>KAVIDIDAATKIMCSNAKAISLNEVEKNEIISKYREITAKKSERAELKEVEPIPLDWPSDLTLPPLPESTNDYVWAGKRKELDDYPRKQLIIDGLSIVIPTYNRAKILAITLACLCNQKTIYDYEVIVADDGSKENIEE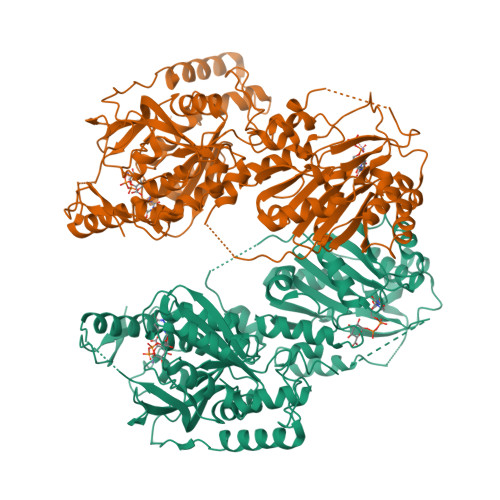IVREFESLLNIKYVRQKDYGYQLCAVRNLGLRAAKYNYVAILDCDMAPNPLWVQSYMELLAVDDNVALIGPRKYIDTSKHTYLDFLSQKSLINEIPEIITNNQVAGKVEQNKSVDWRIEHFKNTDNLRLCNTPFRFFSGGNVAFAKKWLFRAGWFDEEFTHWGGEDNEFGYRLYREGCYFRSVEGAMAYHQEPPGKENETDRAAGKNITVQLLQQKVPYFYRKKEKIESATLKRVPLVSIYIPAYNCSKYIVRCVESALNQTITDLEVCICDDGSTDDTLRILQEHYANHPRVRFISQKNKGIGSASNTAVRLCRGFYIGQLDSDDFLEPDAVELCLDEFRKDLSLACVYTTNRNIDREGNLISNGYNWPIYSREKLTSAMICHHFRMFTARAWNLTEGFNESISNAVDYDMYLKLSEVGPFKHINKICYNRVLHGENTSIKKLDIQKENHFKVVNESLSRLGIKKYKYSPLTNLNECRKYTWEKI[4x]> MEQPYVYAYPQGSGPSGAPT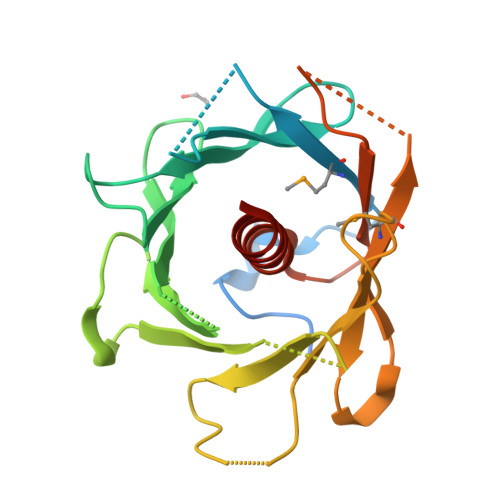PQAGGVVVDPKYCAPYPIDMAIVRKMMSLTDGNFVITDVNGNLLFKVKEPVFGLHDKRVLLDGSGTPVVTLREKMVSMHDRWQVFRGGSTDQRDLLYTVKRSSMLQLKTKLDVFLGHNKDEKRCDFRVKGSWLERSCVVYAGESDAIVAQMHRKHTVQSVFLGKDNFSVTVYPNVDYAFIASLVVILDDVNREDRAA>MGSSHHHHHHSQDPNSMTTLTRQDLNFGQVVADVLCEFLEVAVHLILYVREVYPVGIFQKRKKYNVPVQMSCHPELNQYIQDTLHCVKPLLEKNDVEKVVVVILDKEHRPVEKFVFEITQPPLLSISSDSLLSHVEQLLAAFILKISVCDAVLDHNPPGCTFTVLVHTREAATRNMEKIQVIKDFPWILADEQDVHMHDPRLIPLKTMTSDILKMQLYVEERAHKGSGSGSGSGSGSH[2x];>[2x]MLTPTPDSSPRSTSSPSQSKNGSFTPRTANILKPLMSPPSREEIMATLLDHD;>MLKHEGPPAEKPLEELSASTSGVPGLSSL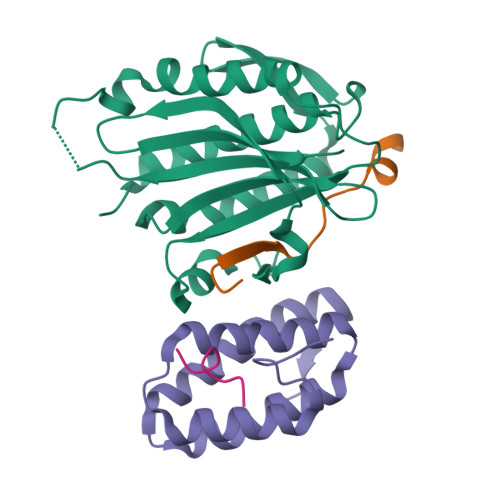QSDPAGCVRPPAPNLAGAVEFNDVKTLLREWITTISDPMEEDILQVVKYCTDLIEEKDLEKLDLVIKYMKRLMQQSVESVWNMAFDFILDNVQVVLQQTYGSTLKVT[2x];> KKSFFDKKRS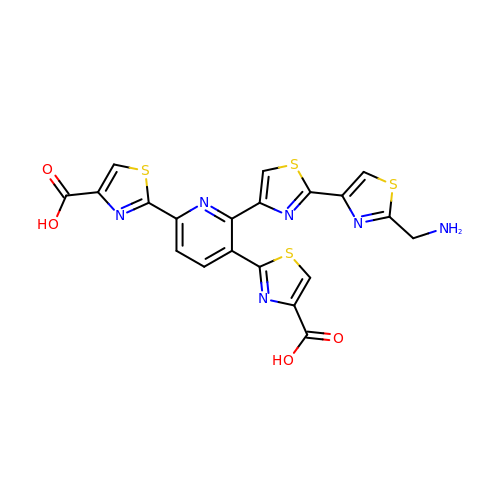2,2'-(6-(2'-(aminomethyl)-[2,4'-bithiazol]-4-yl)pyridine-2,5-diyl)bis(thiazole-4-carboxylic acid) | C20 H12 N6 O4 S4 | YMFHXIFIYXCKLO-UHFFFAOYSA-N>ASCFALISGTANQVKCYRFRVKKNHRHRYENCTTTWFTVADNGAERQGQAQILITFGSPSQRQDFLKHVPLPPGM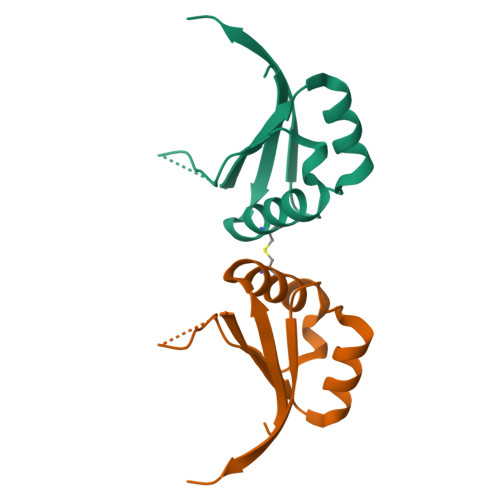NISGFTASLDF[3x]> MAFEALTGINGDLITRSWSASKQAYLTERYHKEEAGAVVIFAFQPSFSEKDFFDPDNKSSFGEIKLNRVQFPCMRKIGKGDVATVNEAFLKNLEAIIDPRTSFQASVEMAVRSRKQIVFTGHSSGGATAILATVWYLEKYFIRNPNVYLEPRCVTFGAPLVGDSIFSHALGREK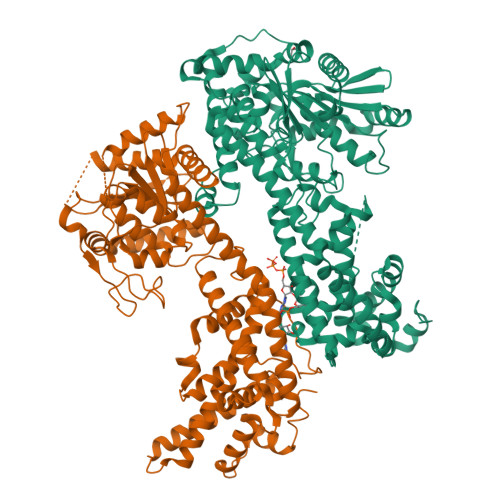WSRFFVNFVSRFDIVPRIMLARKASVEETLPHVLAQLDPRKSSVQESEQRITEFYTRVMRDTSTVANQAVCELTGSAEAFLETLSSFLELSPYRPAGTFVFSTEKRLVAVNNSDAILQMLFYTSQASDEQEWSLIPFRSIRDHHSYEELVQSMGKKLFNHLDGENSIESTLNDLGVSTRGRQYVQAALEEEKKRVENQKKIIQVIEQERFLKKLAWIEDEYKPKCQAHKNGYYDSFKVSNEENDFKANVKRAELAGVFDEVLGLMKKCQLPDEFEGDIDWIKLATRYRRLVEPLDIANYHRHLKNEDTGPYMKRGRPTRYIYAQRGYEHYILKPNGMIAEDVFWNKVNGLNLGLQLEEIQETLKNSGSECGSCFWAEVEELKGKPYEEVEVRVKTLEGMLGEWITDGEVDDKEIFLEGSTFRKWWITLPKNHKSHSPLRDYMMDEITDT;> MESSSSLKGSALGKLVVTSGLLHSSWSKILEIHNPPYSNHDPGLQVSKKKKDSGLEFQIHREEKFTLVVFSAPPICRSSSSDSTLLHVKDKENPFPFLCSENNPSFSLHTPAFNLFTSASTSLTYLKSELLQTLKSEKPVIITGAALGGSVASLYTLWLLETIEPTLKRPLCITFGSPLIGDASLQQILENSVRNSCFLHVVSAQTRIKMDFFKPFGTFLICFDSGCVCIEDHVAVTELLNGVHDSGLVDYSQVLNRLDQSMLSLADSRLIPEDVIKGIEKRAEMKNLRFDMMFKKLNDMKISMAYIEWYKKKCKEVKIGYYDRFKTQLAFPSKEFDINIKNHHKSELNRFWKSVVEEVERRPQSDASILKRRFLFSGNNYRRMIEPLDIAEYYLEGRKEYRTTGRSHHYVMLEKWFGMESILIEKERCKKRDLSDLLTFDSCFWAEVEDSLIVINQLNTTVGMRDDVREVLTRKLVEFEGYVWEIITKREVSPEIFLEESSFMKWWKEYKKIKGFNSSYLTEFMNTRKYESYGKSQ>XGEFAQALKEFAKALKEFAW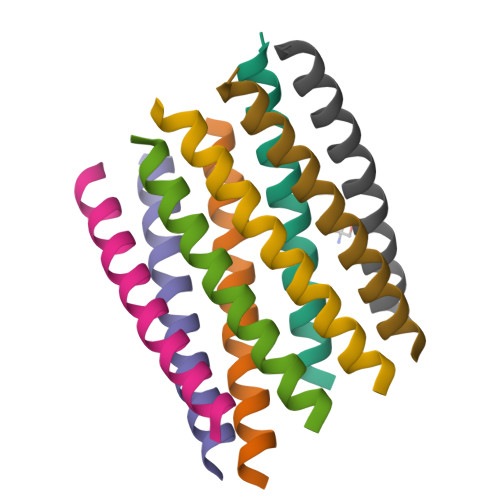ALKEFAQALKGX[8x]>[4x]MGGSHHHHHHSSGENLYFQGHMVLLHMKRSELDQFLFETTVASTVDETTRQMAEVHNLRHRIERLKAEGEELAKHGPAKRPDQQGIDRYQEAPVEKGPNYAEDPTG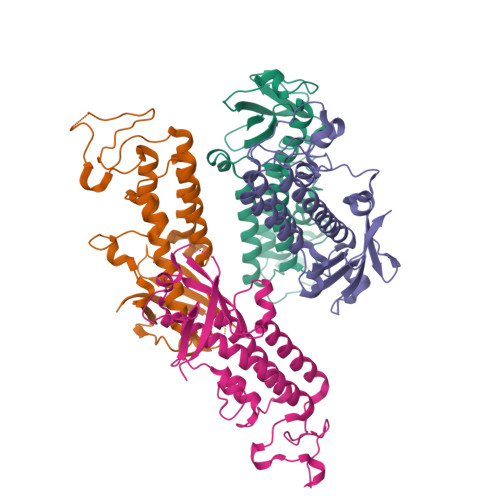RRTGNACDPEVAKVLVKTLEEAVAVAHKDQVAKKMPLTIKALQEAVDNVRGAVMICYPMGLPEWDPVRLGLEGSEDLAGTSYAADELPADVATLWFAGKQMAPEKKLSDYLGRHEKTKAVVKLQKKGQGAPSR> GPMASSENASSAKLSVPERQKLAQQSAGKVLTLLDLSEVQLDGAATLVLTFSIPLDPDQDFSRVIHVVDKKSGKVDGAWELSDNLKELRLRHLEPKRDLIVTIGKEVKALNNATFSKDYEKTITTRDIQPSVGFASRGSLLPGKVVEGLPVMALNVNNVDVNFFRVKPESLPAFISQWEYRNSLANWQSDKLLQMADLVYTGRFDLNPARNTREKLLLPLGDIKPLQQAGVYLAVMNQAGRYDYSNPATLFTLSDIGVSAHRYHNRLDIFTQSLENGAAQQGIEVSLLNEKGQTLTQATSDAQGHVQLENDKNAALLLARKDGQTTLLDLKLPALDLAEFNIAGAPGYSKQFFMFGPRDLYRPGETVILNGLLRDADGKALPNQPIKLDVIKPDGQVLRSVVSQPENGLYHFTWPLDSNAATGMWHIRANTGDNQYRMWDFHVEDFMPERMALNLTGEKTPLTPKDEVKFSVVGYYLYGAPANGNTLQGQLFLRPLREAVSALPGFEFGDIAAENLSRTLDEVQLTLDDKGRGEVSTESQWKETHSPLQVIFQGSLLESGGRPVTRRAEQAIWPADALPGIRPQFASKSVYDYRTDSTVKQPIVDEGSNAAFDIVYSDAQGVKKAVSGLQVRLIRERRDYYWNWSEDEGWQSQFDQKDLIENEQTLDLKADETGKVSFPVEWGAYRLEVKAPNEAVSSVRFWAGYSWQDNSDGSGAVRPDRVTLKLDKASYRPGDTIKLHIAA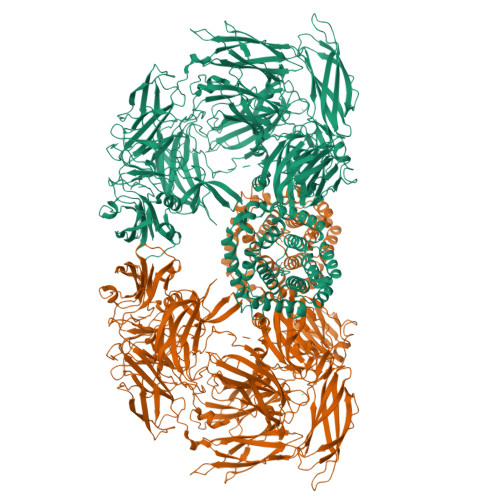PTAGKGYAMVESSEGPLWWQEIDVRAQGLDLTIPVDKTWNRHDLYLSTLVVRPGDKSRSATPKRAVGVLHLPLGDENRRLDLALETPAKMRPNQPLTVKIKASTKNGEKPKQVNVLVSAVDSGVLNITDYVTPDPWQAFFGQKRYGADIYDIYGQVIEGQGRLAALRFGGDGDELKRGGKPPVNHVNIVVQQALPVTLNEQGEGSVTLPIGDFNGELRVMAQAWTADDFGSNESKVIVAAPVIAELNMPRFMASGDTSRLTLDITNLTDKPQKLNVALTASGLLELVSDSPAAVELAPGVRTTLFIPVRALPGYGDGEIQATISGLALPGETVADQHKQWKIGVRPAFPAQTVNYGTALQPGETWAIPADGLQNFSPVTLEGQLLLSGKPPLNIARYIKELKAYPYGCLEQTASGLFPSLYTNAAQLQALGIKGDSDEKRRASVDIGISRLLQMQRDNGGFALWDKNGDEEYWLTAYVMDFLVRAGEQGYSVPTDAINRGNERLLRYLQDPGMMSIPYADNLKASKFAVQSYAALVLARQQKAPLGALREIWEHRADAASGLPLLQLGVALKTMGDATRGEEAIALALKTPRNSDERIWLGDYGSSLRDNALMLSLLEENKLLPDEQYTLLNTLSQQAFGERWLSTQESNALFLAARTIQDLPGKWQAQTSFSAEQLTGEKAQNSNLNSDQLVTLQVSNSGDQPLWLRMDASGYPQSAPLPANNVLQIERHILGTDGKSKSLDSLRSGDLVLVWLQVKASNSVPDALVVDLLPAGLELENQNLANGSASLEQSGGEVQNLLNQMQQASIKHIEFRDDRFVAAVAVDEYQPVTLVYLARAVTPGTYQVPQPMVESMYVPQWRATGAAEDLLIVRP>MHHHHHHELYLDTSDVVAVKALSRIFPLAGVTTNPSIIAAGKKPLDVVLPQLHEAMGGQGRLFAEVMATTAEGMVNDALKLRSIIADIVVKVPVTAEGLAAIKMLKAEGIPTLGTAVYGAAQGLLSALAGAEYVAPFVNRIDAQGGSGIQTVTDLHQLLKMHAPQAKVLAASFKTPRQALDCLLAGCESITLPLDVAQQMISYPAVDA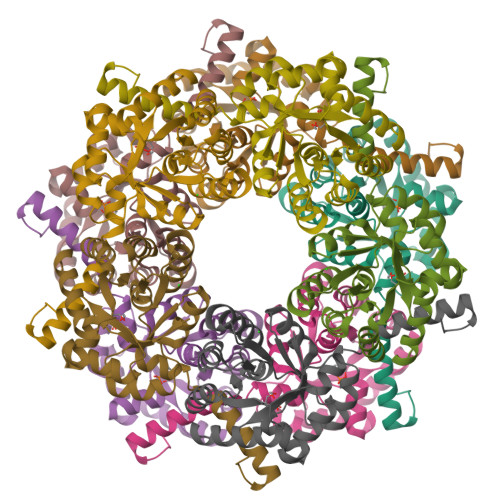AVAKFEQDWQGAFGRTSI[10x]S1 nuclease from Aspergillus oryzae (EC 3.1.30.1; NCBI sequence ID: XP_001818636; S1–P1 nuclease family in Pfam, PF02265) is an extracellular, single–strand–specific, sugar non–specific, Zn2+–dependent, fungal nuclease with 3'–mononucleotidase activity with a pH optimum in range 4.0–4.3. S1 nuclease has the phospholipase C/P1 nuclease–like fold stabilized by two disulfide bridges. The active site is located in a surface cleft and composed of the obligatory catalytic trinuclear zinc cluster supplemented by Lys68 and the nucleoside binding site 1 (NBS1; also called Phe site in the previous studies). A cluster of three zinc ions coordinates the substrate/product scissile phosphate and the reaction mechanism utilizes water activated by Zn2+ ions as a nucleophile.

Each of the two protein chains in the asymmetric unit binds one phosphate and one molecule of adenosine 5'–monophosphate (5’AMP) in the same binding mode. Phosphate is one product of the 3’–mononucleotidase activity, 5’AMP is a product of nuclease activity. Phosphate is present inside the zinc cluster, 5’AMP occupies the NBS1 site in an inverted orientation with respect to the standard substrate/product binding (the ribose moiety is far from the zinc cluster). One of the phosphate oxygen atoms replaces the water molecule W1 and binds almost symmetrically between Zn1 and Zn2. Another oxygen atom binds asymmetrically between Zn1 and Zn3 replacing W2. The phosphate moiety of 5’AMP interacts not with the zinc cluster but instead with Asp83Oδ2 of NBS1 through a sodium ion. The adenine base binds inside NBS1 in a position almost exactly above and parallel to the side chain of Phe81. The water molecule WNBS1 is substituted by the amino group of the adenine base, which enables a deeper penetration of the ligand, and therefore we denote this binding mode as deep. Hydrogen bonding to Asp83 is realized through the Hoogsteen face of adenine.

>WGNLGHETVAYIAQSFVASSTESFCQNILGDDSTSYLANVATWADTYKYTDAGEFSKPYHFIDAQDNPPQSCGVDYDRDCGSAGCSISAIQNYTNILLESPNGSEALNALKFVVHIIGDIHQPLHDENLEAGGNGIDVTYDGETTNLHHIWDTNMPEEAAGGYSLSVAKTYADLLTERIKTGTYSSKKDSWTDGIDIKDPVSTSMIWAADANTYVCSTVLDDGLAYINSTDLSGEYYDKSQPVFEELIAKAGYRLAAWLDLIASQPS[2x]>KHQVFPSFHGADVRKTILSHILESFRRKGIDPFIDNNIERSKSIGHELKEAIKGSKIAIVLLSKNYASSSWCLDELAEIMKCRELLGQIVMTIFYEVDPTDIKKQTGEFGKAFTKTCKGKTKEYVERWRKALEDVATIAGYHSHKWRNEADMIEKIATDVSNMLN[2x];>[2x]KHHVFPSFHGADVRKTILSHILESFRRKGIDPFIDNNIERSKSIGHELKEAIKGSKIAIVLLSKNYASSSWCLDELAEIMKCRELLGQIVMTIFYEVDPTDIKKQTGEFGKAFTKTC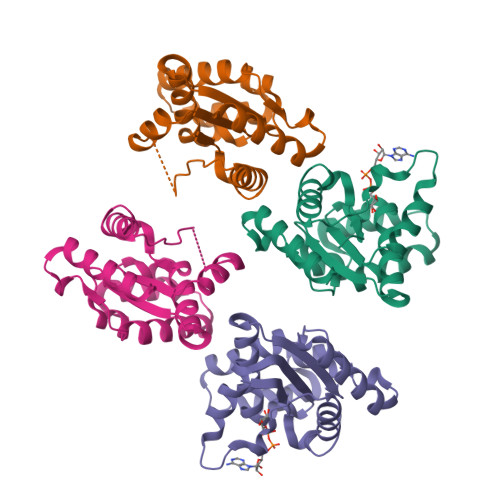KGKTKEYVERWRKALEDVATIAGYHSHKWRNEADMIEKIATDVSNMLN>[3x]MNGKFADGPYSGILDSVLDAIGNTPMVRMKRLAKVYGLECDLLAKCEFMSAGGSVKDRIGKAMVEKAEREGRLKAGDTLIEPTSGNTGIGLALAAAVRGYRMIVTMPAKMSAEKSNIMKCLGAEIVRTPTEAAWNDENSHMGVAAKLQRELENAHILDQYNNTANPMVHYDVTAEEIITQCDGDIDMVVIGAGTGGTITGIGRKIKERCPKCKVVGVDPKGSILAVPDSLNDEKRLQSYEVEGIGYDFVPGVLDRKVVDEWVKVGDAESFTTARAIIRNEGLFVGGSSGANVWGALQAARQLKKGQKCVVLLPDSSRNYMSKFISDEWMAE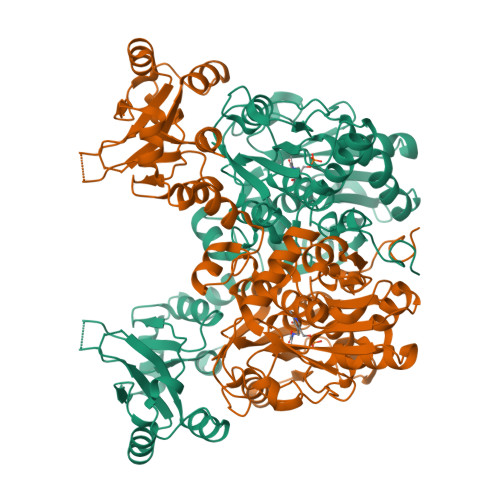HGFAPEDGAKVKEREKQFGGARIRDLLSETGATSDVPFVTARLSVEDVIKMMHETKVKEVIVTEDSEADGKTKLVGVLSEDHIAHSLQSGRCAMQSPVKDIAFKKLAKALPSAYLRDVAKALDFSPYVCVMDEKPSTKKQAGMGEHERAKISLRKAGNSRECPHFLGVITRIDLLHWLATKQK> MSEFFPVPKPIKLNPHVELEVFQCQDTIFQLSVIAPNAKLESHQHPESQIGMVLSGELELYI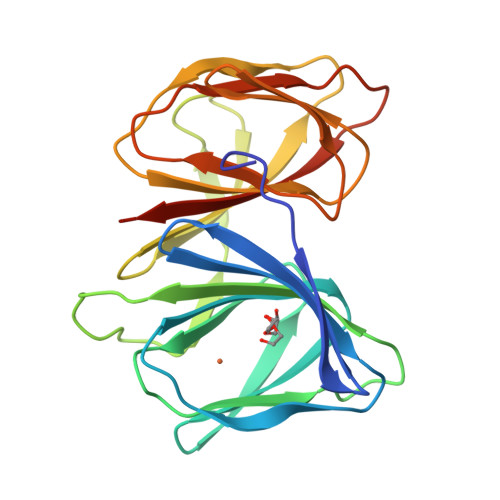KDVIKPLRALQDIHVADANVSHGFVNPLSEPMIGFDLKRITSSLPSEDVVLTLSNNQDKITHLPCQSVKGSWFEIVMMKIPSGYSIPPHQGEQEEIGFILNGKLEIFIENEEQCLEYGQIYYAPSKVLKKGYNSSNQDINLIKILILEHHHHHH[[(2~{R},3~{S},4~{R},5~{R})-5-[2,6-bis(azanyl)purin-9-yl]-3,4-bis(oxidanyl)oxolan-2-yl]methoxy-oxidanyl-phosphoryl] phosphono hydrogen phosphate | C10 H17 N6 O13 P3 | 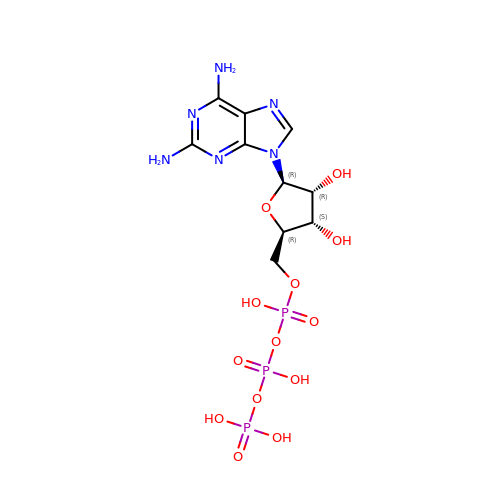CABDYDUZLRXGTB-UUOKFMHZSA-N>[2x]MAHHHHHHSLGLMIKTAECRA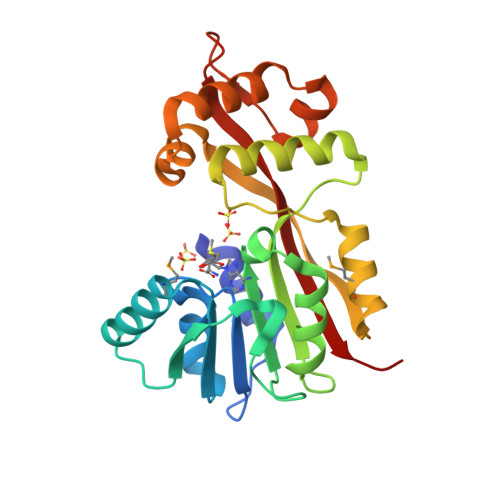EHRVLDIGAGAGHTALAFSPYVQECIGVDATKEMVEVASSFAQEKGVENVRFQQGTAESLPFPDDSFDIITCRYAAHHFSDVRKAVREVARVLKQDGRFLLVDHYAPEDPVLDEFVNHLNRLRDPSHVRESSLSEWQAMFSANQLAYQDIQKWNLPIQYDSWIKRGGTPADREKQIITHLNHASDEARDTFCITLNQNGQPISFCLKAILIQGIKREG>[2x]NPYDVVVIGGGPGGYVASIKAAQLGMKTACVEKRGALGGTCLNVGCIPSKALLHATHLYHDAHANFARYGLMGGEGVTMDSAKMQQQKERAVKGLTGGVEYLFKKNKVTYYKGEGSFETAHSIRVNGLDGKQEMLET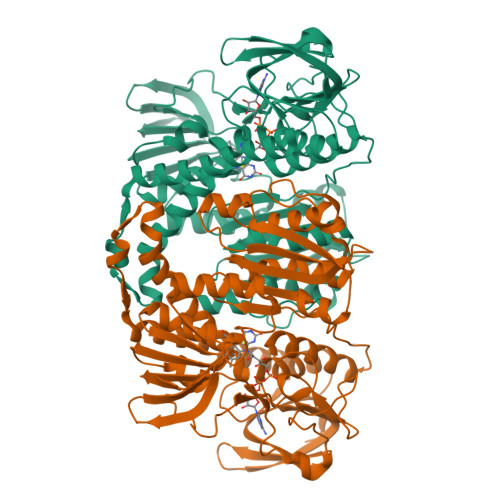KKTIIATGSEPTELPFLPFDEKVVLSSTGALALPRVPKTMVVIGGGVIGLELGSVWARLGAEVTVVEFAPRCAPTLDEDVTNALVGALAKNEKMKFMTSTKVVGGTNNGDSVSLEVEGKNGKRETVTCEALLVSVGRRPFTGGLGLDKINVAKNERGFVKIGDHFETSIPDVYAIGDVVDKGPMLAHKAEDEGVACAEILAGKPGHVNYGVIPAVIYTMPEVASVGKSEDELKKEGVAYKVGKFPFNANSRAKAVSTEDGFVKVLVDKATDRILGVHIVCTTAGELIGEACLAMEYGASSEDVGRTCHAHPTMSEALKEACMALFAKTINF> SSLDDKPQFPGASAEFIDKLEFIQPNVISGIPIYRVMDRQGQIINPSEDPHLPKEKVLKLYKSMTLLNTMDRILYESQRQGRISFYMTNYGEEGTHVGSAAALDNTDLVFGQYREAGVLMYRDYPLELFMAQCYGNISDLGKGRQMPVHYGCKERHFVTISSPL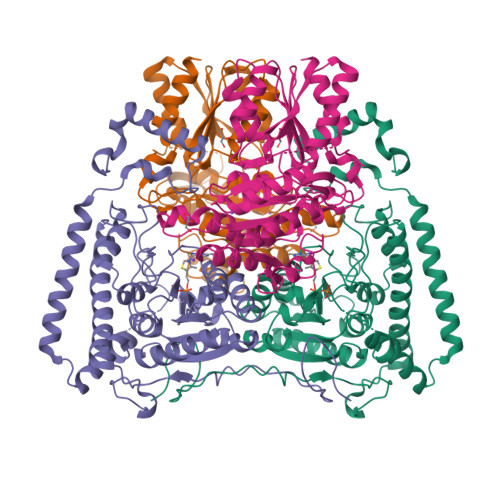ATQIPQAVGAAYAAKRANANRVVICYFGEGAASEGDAHAGFNFAATLECPIIFFCRNNGYAISTPTSEQYRGDGIAARGPGYGIMSIRVDGNDVFAVYNATKEARRRAVAENQPFLIEAMTYRIGHHSTSDDSSAYRSVDEVNYWDKQDHPISRLRHYLLSQGWWDEEQEKAWRKQSRRKVMEAFEQAERKPKPNPNLLFSDVYQEMPAQLRKQQESLARHLQTYGEHYPLDHFDK;> VAHFTFQPDPEPREYGQTQKMNLFQSVTSALDNSLAKDPTAVIFGEDVAFGGVFRCTVGLRDKYGKDRVFNTPLCEQGIVGFGIGIAVTGATAIAEIQFADYIFPAFDQIVNEAAKYRYRSGDLFNCGSLTIRSPWGCVGHGALYASQSPEAFFAHCPGIKVVIPRSPFQAKGLLLSCIEDKNPCIFFEPKILYRAAAEEVPIEPYNIPLSQAEVIQEGSDVTLVAWGTQVHVIREVASMAKEKLGVSCEVIDLRTIIPWDVDTICKSVIKTGRLLISHEAPLTGGFASEISSTVQEECFLNLEAPISRVCGYDTPFPHIFEPFYIPDKWKCYDALRKMINY4-~{tert}-butyl-~{N}-[2-methyl-3-[6-[4-(4-methylpiperazin-1-yl)carbonylphenyl]-7~{H}-pyrrolo[2,3-d]pyrimidin-4-yl]phenyl]benzamide 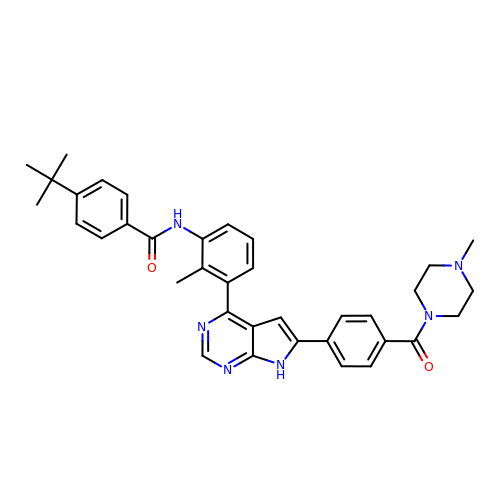| C36 H38 N6 O2 | IGVLLOMIUXKXBM-UHFFFAOYSA-N> RNILRNDEGLYGGQSLDVNPYHFIMQEDCNLVLYDHSTSVWASNTGILGKKGCRAVLQSDGNFVVYDAEGRSLWASHSVRGNGNYVLVLQEDGNVV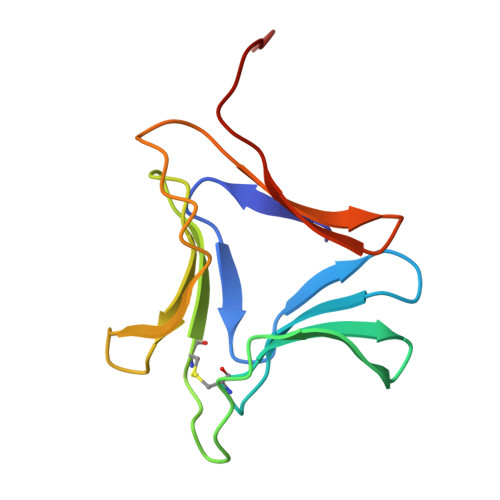IYRSDIWSTN>MNMTNNQSNDFVVIKAVEDGVNVIGLTRGTDTRFHHSEKLDKGEVMICQFTEHTSAIKVRGEALIQTANGEMKSESKK[2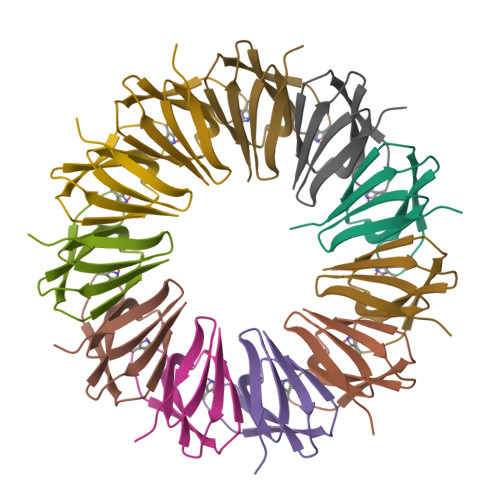2x]> MFNRTTQLKSKHPCSVCTRRKVKCDRMIPCGNCRKRGQDSECMKSTKLITASSSKEYLPDLLLFWQNYEYWITNIGLYKTKQRDLTRTPANLDTDTEECMFWMNYLQKDQSFQLMNFAMENLGALYFGSIGDISELYLRVEQYWDRRAD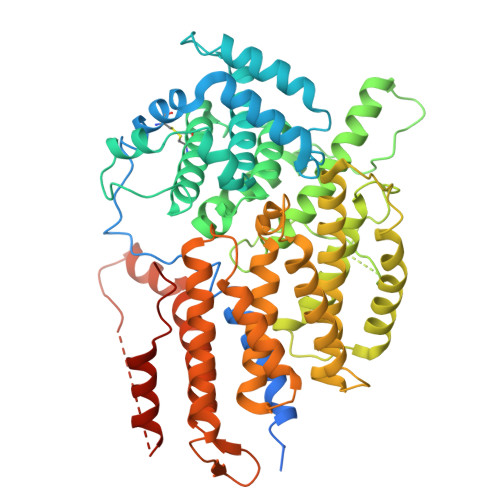KNHSVDGKYWDALIWSVFTMCIYYMPVEKLAEIFSVYPLHEYLGSNKRLNWEDGMQLVMCQNFARCSLFQLKQCDFMAHPDIRLVQAYLILATTTFPYDEPLLANSLLTQCIHTFKNFHVDDFRPLLNDDPVESIAKVTLGRIFYRLCGCDYLQSGPRKPIALHTEVSSLLQHAAYLQDLPNVDVYREENSTEVLYWKIISLDRDLDQYLNKSSKPPLKTLDAIRRELDIFQYKVDSLEEDFRSNNSRFQKFIALFQISTVSWKLFKMYLIYYDTADSLLKVIHYSKVIISLIVNNFHAKSEFFNRHPMVMQTITRVVSFISFYQIFVESAAVKQLLVDLTELTANLPTIFGSKLDKLVYLTERLSKLKLLWDKVQLLDSGDSFYHPVFKILQNDIKIIELKNDEMFSLIKGLGSLVPLNKLRQESLLEEEDENNTEPSDFRTIVEEFQSEYNISDILSGSGGSGENLYFQ> GEKRKSRQAEVNIGMVGHVDHGKTTLTKALTGVWTDTHSEELRRGITIKIGFADAEIRRCPNCGRYSTSPVCPYCGHETEFVRRVSFIDAPGHEALMTTMLAGASLMDGAILVIAANEPCPRPQTREHLMALQIIGQKNIIIAQNKIELVDKEKALENYRQIKEFIEGTVAENAPIIPISALHGANIDVLVKAIED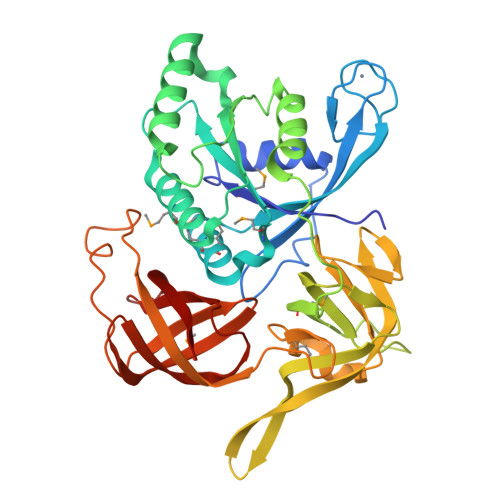FIPTPKRDPNKPPKMLVLRSFDVNKPGTPPEKLVGGVLGGSIVQGKLKVGDEIEIRPGVPYEEHGRIKYEPITTEIVSLQAGGQFVEEAYPGGLVGVGTKLDPYLTKGDLMAGNVVGKPGKLPPVWDSLRLEVHLLERVVGTEQELKVEPIKRKEVLLLNVGTARTMGLVTGLGKDEIEVKLQIPVCAEPGDRVAISRQIGSRWRLIGYGIIKE> MAGLNEILLPEVHLNSPIVRYKLFYYILHGQLPNDLEPDDLGPLANQNWKAIRAEESQVHARLKQIRVELIARIPSLRWTRSQREIAILIWPRILPILQAYDLRQSMQLPTVWEKLTQSTVNLISDGLERVVLHISNQLTGKPNLFTRSRAGQDTKDYSIPSTRELSQIWFNNEWSGSVKTWLMIKYRMRQLITNQKTGELTDLVTIVDTRSTLCIITPELVALYSSEHKALTYLTFEMVLMVTDMLEGRLNVSSLCTASHYLSPLKKRIEVLLTLVDDLALLMGDKVYGIVSSLESFVYAQLQYGDPVIDIKGTFYGFICNEILDLLTEDNIFTEEEANKVLLDLTSQFDNLSPDLTAELLCIMRLWGHPTLTASQAASKVRESMCAPKVLDFQTIMKTLAFFHAILINGYRRSHNGIWPPTTLHGNAPKSLIEMRHDNSELKYEYVLKNWKSISMLRIHKCFDASPDEDLSIFMKDKAISCPRQDWMGVFRRSLIKQRYRDANRPLPQPFNRRLLLNFLEDDRFDPIKELEYVTSGEYLRDPEFCASYSLKEKEIKATGRIFAKMTKRMRSCQVIAESLLANHAGKLMRENGVVLDQLKLTKSLLTMNQIGIISEHSRRSTADNMTLAHSGSNKHRINNSQFKKNKDNKHEMPDDGFEIAACFLTTDLTKYCLNWRYQVIIPFARTLNSMYGIPHLFEWIHLRLMRSTLYVGDPFNPPSDPTQLDLDTALNDDIFIVSPRGGIEGLCQKLWTMISISTIILSATEANTRVMSMVQGDNQAIAITTRVVRSLSHSEKKEQAYKASKLFFERLRANNHGIGHHLKEQETILSSDFFIYSKRVFYKGRILTQALKNVSKMCLTADILGDCSQASCSNLATTVMRLTENGVEKDLCYFLNAFMTIRQLCYDLVFPQTKSLSQDITNAYLNHPILISRLCLLPSQLGGLNFLSCSRLFNRNIGDPLVSAIADVKRLIKAGCLDIWVLYNILGRRPGKGKWSTLAADPYTLNIDYLVPSTTFLKKHAQYTLMERSVNPMLRGVFSENAAEEEEELAQYLLDREVVMPRVAHVILAQSSCGRRKQIQGYLDSTRTIIRYSLEVRPLSAKKLNTVIEYNLLYLSYNLEIIEKPNIVQPFLNAINVDTCSIDIARSLRKLSWATLLNGRPIEGLETPDPIELVHGCLIIGSDECEHCSSGDDKFTWFFLPKGIRLDDDPASNPPIRVPYIGSKTDERRVASMAYIKGASVSLKSALRLAGVYIWAFGDTEESWQDAYELASTRVNLTLEQLQSLTPLPTSANLVHRLDDGTTQLKFTPASSYAFSSFVHISNDCQILEIDDQVTDSNLIYQQVMITGLALIETWNNPPINFSVYETTLHLHTGSSCCIRPVESCVVNPPLLPVPLINVPQMNKFVYDPEPLSLLEMEKIEDIAYQTRIGGLDQIPLLEKIPLLAHLTAKQMVNSITGLDEATSIMNDAVVQADYTSNWISECCYTYIDSVFVYSGWALLLELSYQMYYLRIQGIQGILDYVYMTLRRIPGMAITGISSTISHPRILRRCINLDVIAPINSPHIASLDYTKLSIDAVMWGTKQVLTNISQGIDYEIVVPSESQLTLSDRVLNLVARKLSLLAIIWANYNYPPKVKGMSPEDKCQALTTHLLQTVEYVEYIQIEKTNIRRMIIEPKLTAYPSNLFYLSRKLLNAIRDSEEGQFLIASYYNSFGYLEPILMESKIFNLSSSESASLTEFDFILNLELSDASLEKYSLPSLLMTAENMDNPFPQPPLHHVLRPLGLSSTSWYKTISVLNYISHMKISDGAHLYLAEGSGASMSLIETFLPGETIWYNSLFNSGENPPQRNFAPLPTQFIESVPYRLIQAGIAAGNGIVQSFYPLWNGNSDITDLSTKTSVEYIIHKVGADTCALVHVDLEGVPGSMNSMLERAQVHALLITVTVLKPGGLLILKASWEPFNRFSFLLTVLWQFFSTIRILRSSYSDPNNHEVYIIATLAVDPTTSSFTTALNRARTLNEQGFSLIPPELVSEYWRKRVEQGQIIQDCIDKVISECVRDQYLADNNIILQAGGTPSTRKWLDLPDYSSFNELQSEMARLITIHLKEVIEILKGQASDHDTLLFTSYNVGPLGKINTILRLIVERILMYTVRNWCILPTQTRLTLRQSIELGEFRLRDVITPMEILKLSPNRKYLKSALNQSTFNHLMGETSDILLNRAYQKRIWKAIGCVIYCFGLLTPDVEGSERIDVDNDIPDYDIHGDII;>MDQFIKQDETGDLIETGMNVANHFLSTPIQGTNSLSKASILPGVAPVLIGNPEQKNIQHPTASHQGSKTKGRGSGVRSIIVSPSEAGNGGTQIPEPLFAQTGQGGIVTTVYQDPTIQPTGSYRSVELAKIGKERMINRFVEKPRTSTPVTEFKRGGPGAAAQGQTIQEEGIDGNGASAGSKERSGSLSGATLYAHLSLPQQDSTPANVGIAPQSAISANEIMDLLRGMDARLQHLEQKVDKVLAQGSMVTQIKNELSTVKTTLATIEGMMATVKIMDPGNPTGVPVDELRRSFSDHVTIVSGPGDVSFSSSEKPTLYLDELARPVSKPRPAKQTKSQPVKDLAGQKVMITKMITDCVANPQMKQAFEQRLAKASTEDALNDIKRDIIRSAI[2x]

L and P function as the RNA polymerase complex, responsible for replicating and transcribing the viral genome. To catalyze the RNA synthesis in both replication and transcription, L sequentially consists of five domains: the RNA-dependent RNA polymerase domain (RdRp), polyribonucleotidyl transferase domain (PRNTase), connector domain (CD), methyltransferase domain (MTase), and C-terminal domain (CTD). P harbors an oligomerization domain (POD) for self-oligomerization, and the oligomeric P attaches to RdRp of L, tethering the polymerase to NC to extract the RNA strand for both replication and transcription. Here, we resolved two L–P complex conformations from the mumps virus (MuV), a typical member of nsNSVs, via cryogenic-electron microscopy.

In cryo-EM maps, four P molecules assemble like a kettle spout stably anchored to L. Our cryo-EM structures capture the clear interface between two P molecules (depicted as P1 and P4, respectively) and L, involving the RdRp, POD, PLinker2, and PCTD regions. Specifically, P1-Met269, P1-Val273, P4-Ala271, and P4-Val273 from the C-terminus of the POD core region, form a hydrophobic cap to trap the conserved residue L-Phe394. A salt bridge between P4-Glu267 and L-Lys453, together with a hydrogen bond between P1-Thr265 and L-Asn428, further stabilizes this interface. The POD tail of P4 folds into a β-strand, forming the anti-parallel β-sheet with Lys390–Asp393 of L. Three electrostatic interactions fix both ends of the β-sheet. Furthermore, L-Gln680 forms hydrogen bonds with P4-Met276 and P4-Asp277, enabling close contact between these two β-strands. Intriguingly, the C-terminal domains of P1 and P4 turn to the template entry side. The turning point occurs at the PLinker2 region of P4 and is trapped in the hydrophobic groove contributed by L-Ala731, L-Leu732, and L-Val739. The PCTD of P4 strides over P1, forming hydrogen bonds among P4-Ser301, L-Arg459, and L-Arg687. Residues from 249 to 299 of P are the major region interacting with L.>[2x]NLFQFEKLIKKMTGKSGMLWYSAYGCYCGWGGQGRPKDATDRCCFVHDCCYGKVTGCN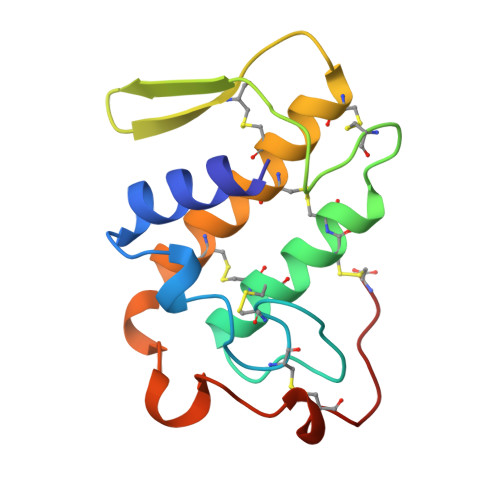PKMDIYTYSVDNGNIVCGGTNPCKKQICECDRAAAICFRDNLKTYDSKTYWKYPKKNCKEESEPC>EEDLTEVKKDALENLRVYLCEKIIAERHFDHLRAKKILSREDTEEISCRTSSRKRAGKLLDYLQENPKGLDTLVES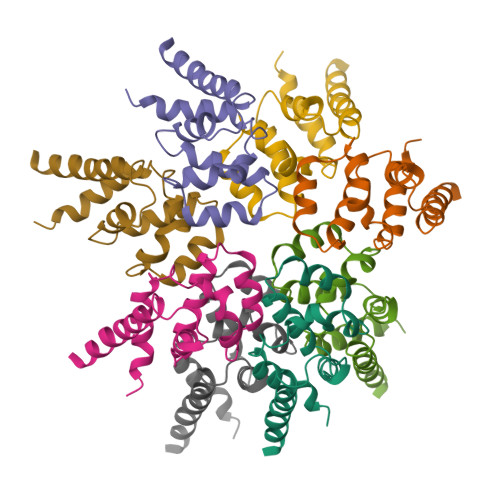IRREKTQNFLIQKITDEVLKLRNIKLEHLK[8x]> MGHQNAAVSENQNHDDGAASSPGFKLVGFSKFVRKNPKSDKFKVKRFHHIEFWCGDATNVARRFSWGLGMRFSAKSDLSTGNMVHASYLLTSGDLRFLFTAPYSPSLSAGEIKPTTTASIPSFDHGSCRSFFSSHGLGVRAVAIEVEDAESAFSISVANGAIPSSPPIVLNEAVTIAEVKLYG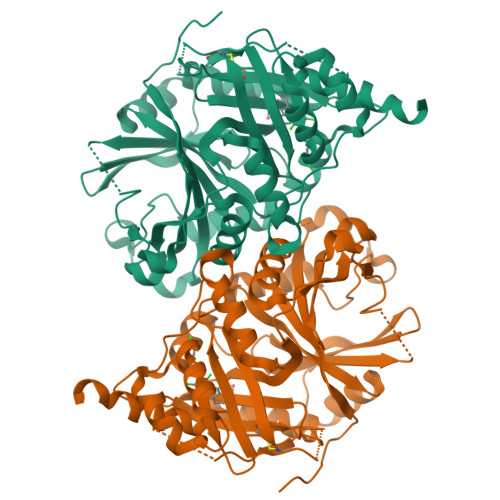DVVLRYVSYKAEDTEKSEFLPGFERVEDASSFPLDYGIRRLDHAVGNVPELGPALTYVAGFTGFHQFAEFTADDVGTAESGLNSAVLASNDEMVLLPINEPVHGTKRKSQIQTYLEHNEGAGLQHLALMSEDIFRTLREMRKRSSIGGFDFMPSPPPTYYQNLKKRVGDVLSDDQIKECEELGILVDRDDQGTLLQIFTKPLGDRPTIFIEIIQRVGCMMKDEEGKAYQSGGCGGFGKGNFSELFKSIEEYEKTLEAKQLVG>[2x]DKVTQSSPDQTVASGSEVVLLCTYDTVYSNPDLFWYRIRPDYSFQFVFYGDDSRSE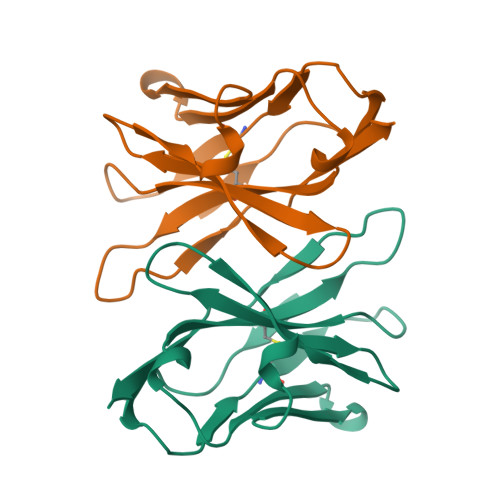GADFTQGRFSVKHILTQKAFHLVISPVRTEDSATYYCAFTLPPPTDKLIFGKGTRVTVEP> MSFVKDFKPQALGDTNLFKPIKIGNNELLHRAVIPPLTRMRALHPGNIPNRDWAVEYYTQRAQRPGTMIITEGAFISPQAGGYDNAPGVWSEEQMVEWTKIFNAIHEKKSFVWVQLLVLGWAAFPDNLARDGLRYDSASDN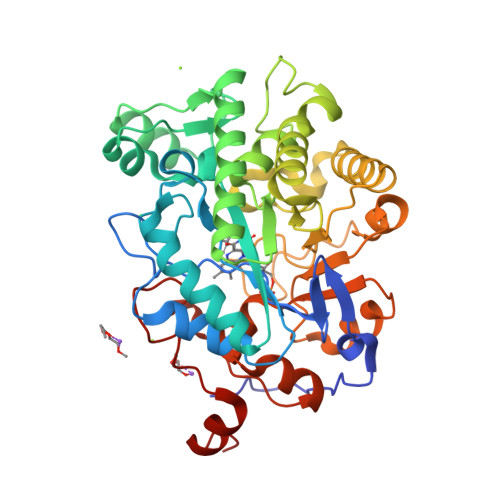VFMDAEQEAKAKKANNPQHSLTKDEIKQYIKEYVQAAKNSIAAGADGVEIHSANGYLLNQFLDPHSNTRTDEYGGSIENRARFTLEVVDALVEAIGHEKVGLRLSPYGVFNSMSGGAETGIVAQYAYVAGELEKRAKAGKRLAFVHLVEPRVTNPFLTEGEGEYEGGSNDFVYSIWKGPVIRAGNFALHPEVVREEVKDKRTLIGYGRFFISNPDLVDRLEKGLPLNKYDRDTFYQMSAHGYIDYPTYEEALKLGWDKK>[2x]MEEPEEPADSGQSLVPVYIYSPEYVSMCDSLAKIPKRASMVHSLIEAYALHKQMRIVKPK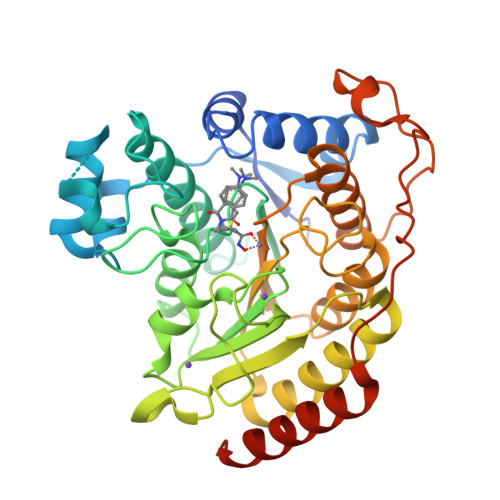VASMEEMATFHTDAYLQHLQKVSQEGDDDHPDSIEYGLGYACPATEGIFDYAAAIGGATITAAQCLIDGMCKVAINWSGGWHHAKKDEASGFCYLNDAVLGILRLRRKFERILYVDLDLHHGDGVEDAFSFTSKVMTVSLHKFSPGFFPGTGDVSDVGLGKGRYYSVNVPIQDGIQDEKYYQICESVLKEVYQAFNPKAVVLQLGADTIAGDPMCSFNMTPVGIGKCLKYILQWQLATLILGGGGYNLANTARCWTYLTGVILGKTLSSEIPDHEFFTAYGPDYVLEITPSCRPDRNEPHRIQQILNYIKGNLKHVVIEGRSHHHHHH> GPLGSEVIQALIFKDDGSL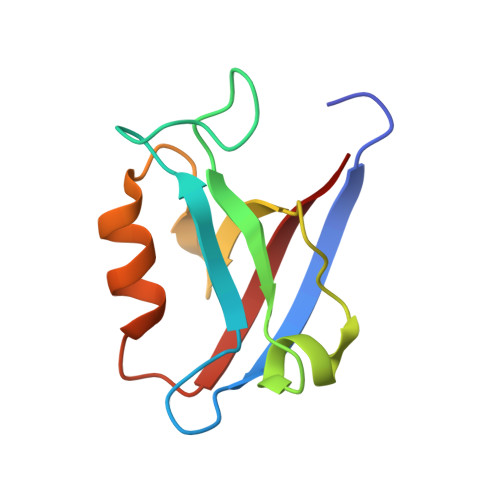GLSISGGVGSSSFKSGDDGIFVSKIAKGGPCDNEGTLKIGDKILSVNEISFTGITHEKAVEILKNQDSKYMVVVERS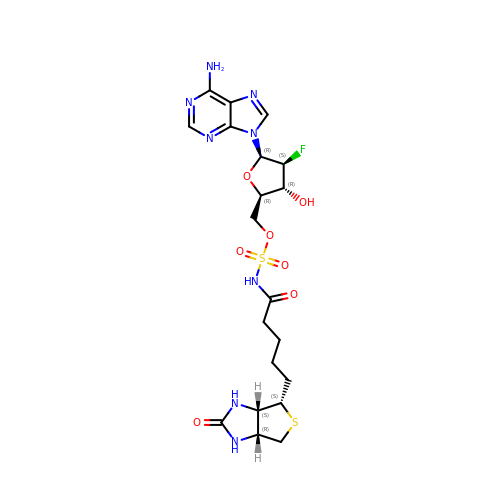9-[2-deoxy-2-fluoro-5-O-({5-[(3aS,4S,6aR)-2-oxohexahydro-1H-thieno[3,4-d]imidazol-4-yl]pentanoyl}sulfamoyl)-beta-D-arabinofuranosyl]-9H-purin-6-amine | C20 H27 F N8 O7 S2 | XTTQQKAKULCXCM-ROPJLRCXSA-N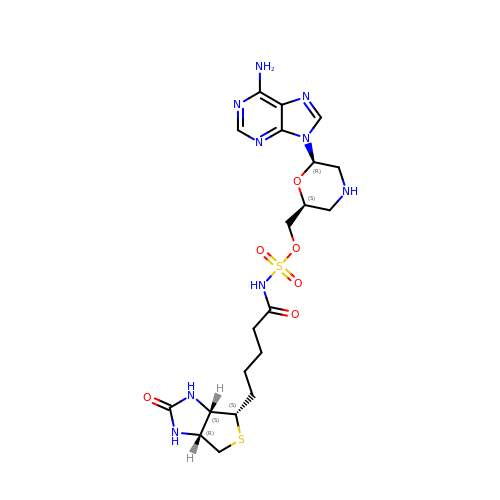[(2S,6R)-6-(6-amino-9H-purin-9-yl)morpholin-2-yl]methyl {5-[(3aS,4S,6aR)-2-oxohexahydro-1H-thieno[3,4-d]imidazol-4-yl]pentanoyl}sulfamate | C20 H29 N9 O6 S2 | IFZKEQZLBVWVDE-RDUHTLEXSA-N>[2x]MSFETLNKSFINGKWTGGESGRTEDILNPYDQSVITTASLATGKQLEDAFDIAQKAQKEWAKSTTEDRKAVLQKARGYLHENRDDIIMMIARETGGTIIKSTIELEQTIAILDEAMTYTGELGGVKEVPSDIEGKTNKIYRLPLGVISSISPFNFPMNLSMRSI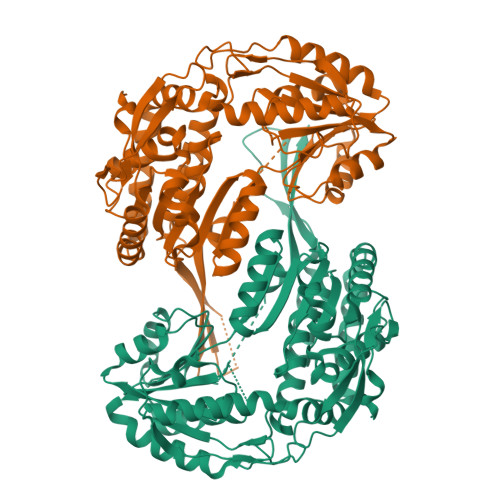APAIALGNSVVHKPDIQTAISGGTIIAKAFEHAGLPAGVLNVMLTDVKEIGDGMLTNPIPRLISFTGSTAVGRHIGEIAGRAFKRMALELGGNNPFAVLSDADVDRAVDAAIFGKFIHQGQICMIINRIIVHQDVYDEFVEKFTARVKQLPYGDQTDPKTVVGPLINERQIEKALEIIEQAKTDGIELAVEGKRVGNVLTPYVFVGADNNSKIAQTELFAPIATIIKAGSDQEAIDMANDTEYGLSSAVFTSDLEKGEKFALQIDSGMTHVNDQSVNDSPNIAFGGNKASGVGRFGNPWVVEEFTVTKWISIQKQYRKYPF>[2x]MPRRDRNMDSAPCMWMRGGTSKGGYFLRADLPADTAARDAFLLAVMGSPDPRQIDGMGGADPLTSKV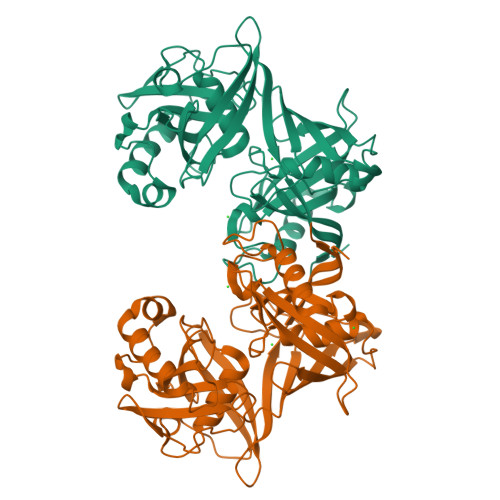AVVSKSERPGIDVDYLFLQVFVDQAIVTDAQNSGNILAGVGPFAIERGLVAASGDETRVAIFMENTGQVAVATVRTPGGSVTYAGDAAIDGVPGTHAPIPTEFRDTAGSSCGALLPSGNAVDVVNGLPVTLIDNGMPCVVMKAADVGITGYEDRDSLDANAELKAKIEAIRLAVGELMNLGDVTEKSVPKMMLVAPPRDGGAVCVRSFIPHRAHATIGVLGAVSVATACLIPGSPAAEVAVVPEGARKTLSIEHPTGEMSCVLEVDDAGNVVSAALLRTARKLMDGVVFVLEHHHHHH2-deoxy-2-fluoro-alpha-D-arabinofuranose 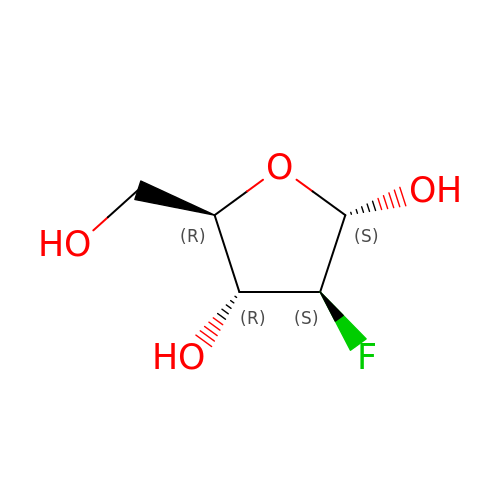| C5 H9 F O4 | RTUWTJAKZMHWBQ-LECHCGJUSA-N> MAGAATATDFPVRRTDLGQVQGLAGDVMSFRGIPYAAPPVGGLRWKPPQHARPWAGVRPATQFGSDCFGAAYLRKGSLAPGVSEDCLYLNVWAPSGAKPGQYPVMVWVYGGGFAGGTAAMPYYDGEALARQGVVVVTFNYRTNILGFFAHPGLSRESPTGTSGNYGLLDILAALRWVQSNARAFGGDPGRVTVFGESAGASAIGLLLTSPLSK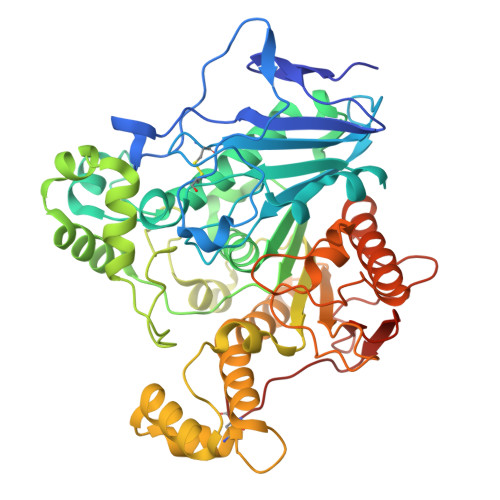GLFRGAILESPGLTRPLATLADSAASGERLDADLSRLRSTDPATLMARADAARPASRDLRRPRPTGPIVDGHVLPQTDSAAIAAGQLAPVRVLIGTNADEGRAFLGRAPMETPADYQAYLEAQFGDQAAAVAACYPLDGRATPKEMVARIFGDNQFNRGVSAFSEALVRQGAPVWRYQFNGNTEGGRAPATHGAEIPYVFGVFKLDELGLFDWPPEGPTPADRALGQLMSSAWVRFAKNGDPAGDALTWPAYSTGKSTMTFGPEGRAAVVSPGPSIPPCADGAKAG>MSSDNIKVIVRCRPLNARETRENALNIIRMDEASAQVIVDPPEQEKSATQAKKVPRTFTFDAVYDQTSCNYGIFQASFKPLIDAVLEGFNSTIFAYGQTGAGKTWTMGGNKEEPGAIPNSFKHLFDAINSSSSNQNFLVIGSYLELYNEEIRDLIKNNTKLPLKEDKTRGIYVDGLSMHRVTTAAELSALMDKGFANRHVAATQMNDTSSRSHSIFMVRIECSEVIENKEVIRVGKLNLVDLAGSERQSKTGATGETLVEGAKINLSLSALGLVISKLVEGATHIPYRDSKLTRLLQDSLGGNSKTLMCANISPASTNYDETMS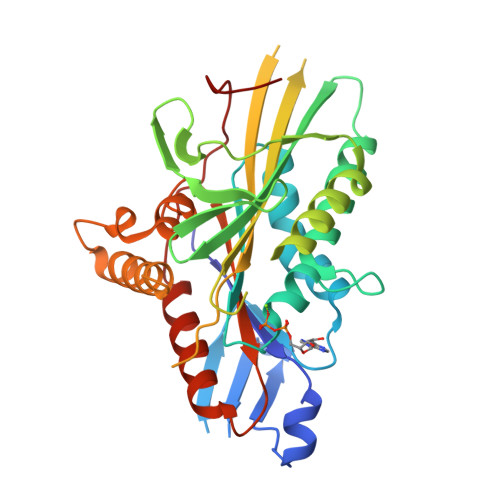TLRYADRAKQIKNKPRINEDPKDAQI[2x]> DKELKFLVVDAFSTMRRIVRNLLK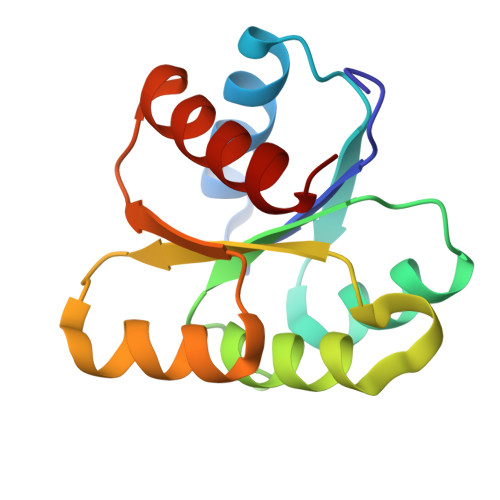ELGFNNVEEAEDGVDALNKLQAGGYGFVISDWNMPNMDGLELLKTIRADGAMSALPVLMVTAEAKKENIIAAAQAGASGYVVKPFTAATLEEKLNKIFEKLGM>GSHMARYDSLLQALGNTPLVGLQRLSPRWDDGRDGPHVRLWAKLEDRNPTGSIKDRPAVRMIEQAEADGLLRPGATILEPTSGNTGISLAMAARLKGYRLICVMPENTSVERRQLLELYGAQIIFSAAEGGSNTAVATAKELAATNPSWVMLYQYGNPANTDSHYCGTGPELLADLPEITHFVAGLGTTGTLMGTGRFLREHVANVKIVAAEPRYGEGVYALRNMDEGFVPELYDPEILTARYSVGAVDAVRRTRELVHTEGIFAGISTGAVLHAALGVGAGALAAGERADIALVVADAGWKYLSTGAYAGS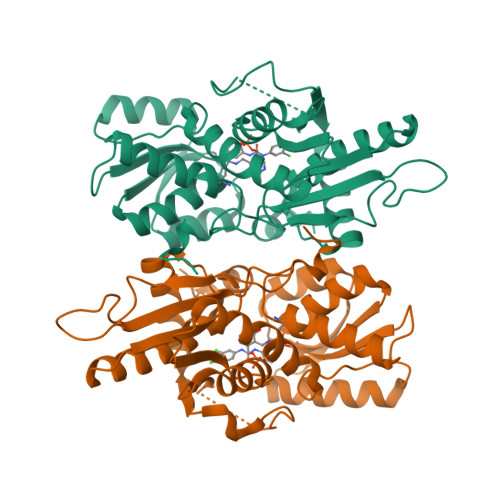LDDAETALEGQLWA[4x]>GSHMMKRLVYVSKISGHLSLEEIQRIGKVSIKNNQRDNITGVLLYLQGLFFQILEGENEKVDKLYKKILVDDRHTNILCLKTEYDITDRMFPNWAMKTINLNENSELMIQPIKSLLQTVTQSHRVLEKYMPARVIYLINQGINPLTVEPQLVEKIIFFSDILAFSTLTEKLPVNEVVILVNRYFSICTRIISAYGGEVTKFIGDCVMASFTKEQGDAAIRTSLDIISELKQLRHHVEATNPLHLLYTGIGLSYGHVIEGNMGSSLKMDHTLLGDAVNVAARLEALTRQLPYALAFTAGVKKCC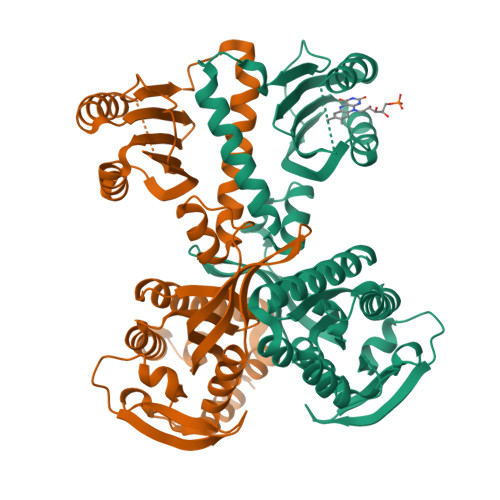QAQWTFINLGAHQVKGKQEAIEVYTVNEAQKYYDTLQITQLIRQTLENDK[2x]>ACGGCGT[4x];>ACGCCGT[4x]

We have determined the crystal structures of DNA duplexes containing -CGCCG- regions as CCG repeat motifs that comprise a non-CpG site with or without cytosine methylation. On the other hand, methylation of cytosines immediately preceding a non-guanine residue is known as non-CpG methylation. Our structural results demonstrated that cytosine methylation at a non-CpG step leads to an anti→syntransition of its complementary guanosine residue toward the (w)cWH geometry as a partial population of WC, in both drug-bound and naked mC:G base pairs. This particular geometry is specific to non-CpG methylated dinucleotide sites in B-form DNA.

To investigate the structural effects of non-CpG methylation on the DNA structure, we have determined the crystal structures of the DNA duplexes d(ACGmCCGT/ACGGCGT) (named as mC:G pairing structure)and d(ACGCCGT/ACGGCGT) (named as C:G pairing structure), which represent methylated and unmethylated states, respectively. These crystal structures have revealed that cytosine methylation at a non-CpG site flanking two CpGs resulted in polymorphic conformations of the central mC:G base pair, including the unexpected formation of a novel water-mediated cis Watson–Crick/Hoogsteen, (w)cWH, base pair arrangement at partial occupancy, which is specific to methylation at a non-CpG site in B-form DNA. On the other hand, six different conformations were observed for mC:G base pairs in the methylated duplexes: In mC:G-NPX1, the mC4: G11 base pair adopts two alternative conformations with occupancy ratios of 0.6 and 0.4, which were designated mC:G-NPX1-1 and mC:G–NPX1-2, respectively. In mC:G-NPX2, mC4:G11 base pair also refined to two alternative conformations with occupancy ratios of 0.9 and 0.1, which were thereby designated mC:G –NPX2-1 and mC:G –NPX2-2, respectively. The central mC4:G11 base pairs of mC:G–NPX3 and mC:G-NPX4 each adopt a WC conformation similar to the unmethylated structure. Interestingly, for mC:G-NPX2, whilst mC4:G11 of mC:G–NPX2-1 adopts an aWC conformation similar to those observed for mC:G–NPX1-1 and mC:G–NPX1-2, the same base pair in mC:G–NPX2-2 adopts anti-syn pairing, in which N4 of mC4 forms a hydrogen bond with O6 of G11. Moreover, a water-mediated hydrogen bond is apparent between O2 of mC4 and N7 of G11. In addition, a bifurcated hydrogen bond was formed between O6 of G11 and protonated N3 of mC4 to further stabilize this anti-synpairing. We have designated the unique geometry observed in mC:G–NPX2-2 as (w)cWH to represent a water-mediated cis Watson–Crick/Hoogsteen base pair geometry. In summary, the base pair geometries of the central mC4:G11 in the methylated duplexes fall into three types: WC (mC:G–NPX3 and mC:G –NPX4), aWC (mC:G–NPX1-1, mC:G–NPX1-2, and mC:G–NPX2-1), and (w)cWH (mC:G–NPX2-2).3-[[4-[[(1~{R})-2,2-dimethyl-1-(5-methylfuran-2-yl)propyl]amino]-1,1-bis(oxidanylidene)-1,2,5-thiadiazol-3-yl]amino]-~{N},~{N},6-trimethyl-2-oxidanyl-benzamide 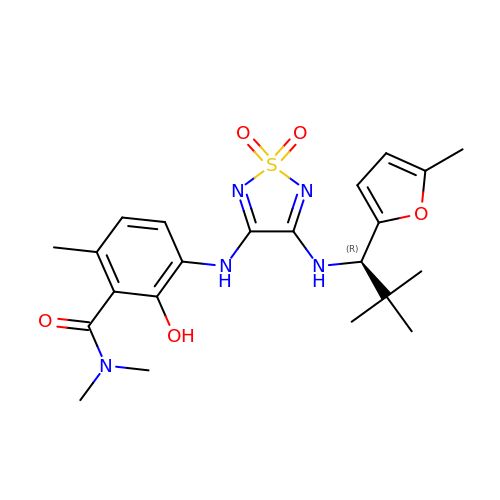| C22 H29 N5 O5 S | MAYXLCLBDVEYAL-SFHVURJKSA-N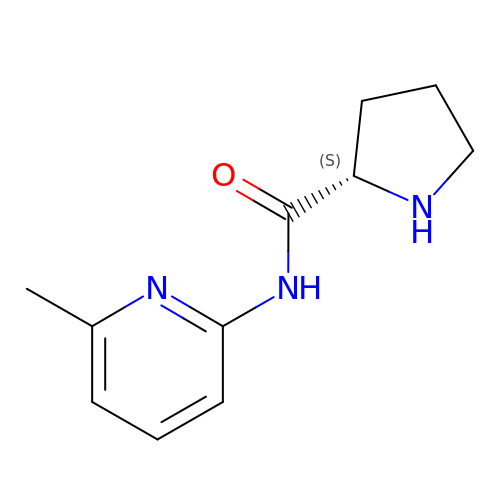N-(6-methylpyridin-2-yl)-L-prolinamide | C11 H15 N3 O | QILVMVSMHKJUDZ-VIFPVBQESA-N> MAAPFDKSKNVAQSIDQLIGQTPALYLNKLNNTKAKVVLKMECENPMASVKDRLGFAIYDKAEKEGKLIPGKSIVVESSSGN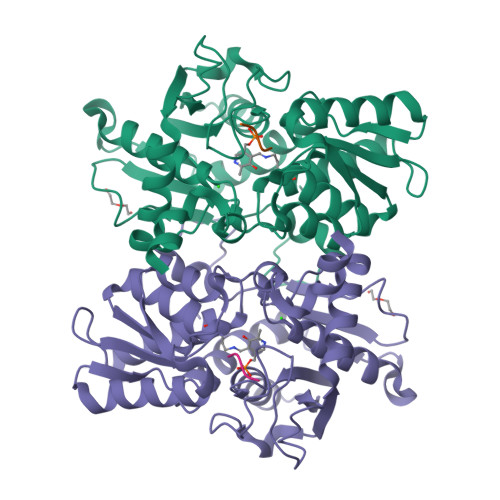TGVSLAHLGAIRGYKVIITMPESMSLERRCLLRIFGAEVILTPAALGMKGAVAMAKKIVAANPNAVLADQFATKYNALIHEETTGPEIWEQTNHNVDCFIAGVGTGGTLTGVARALKKMGSHARIVAVEPTESPVLSGGKPGPHKIQGIGPGFVPDVLDRSLIDEVLCVAGDDAIETALKLTRSDGVFCGFSGGANVYAALKIAERPEMEGKTIVTVIPSFGERYLSTTLYRSVRDEVSSLPVALEHHHHHH;> DWSI>HMASMTGGQQMGRMSHMRPAFGAAWNRFKEVNVNVEQVGKLLGGKVQHNIDAGIF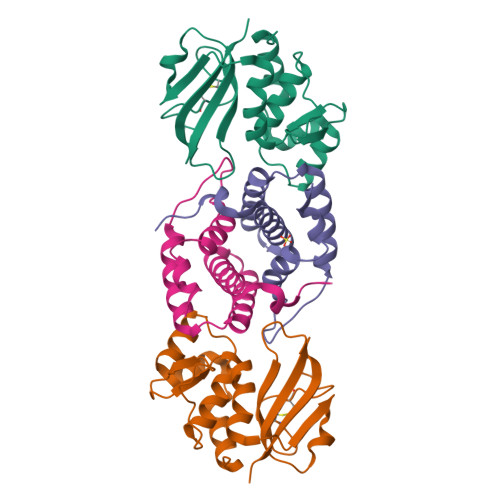KNACPIRMSYVLNYCGIPVPSNSKYATVTGSDKKRYMFRVKDMIAFLPTVLGKADISVSSPTPAQFAGKQGIIIFTGHGWLDATGHVTLWNGNICSDDCHFLGSPGNGSFIPTNATFWSLK[2x];>[2x]QTLPDISTFSQQQIFENWVQNRCIGKIADSKSLKEDADASAAAWLEASNLPAENFEKADEVIVSLLKQKVGGTEPGHYQILKCTLIANSDAIRPLKSSKHHHHHH> IPAGIIPTGNVLSTIEVCAHRCIFDFFKQIRSDDNSLYSAQFDILLGTYCNTLNFVRFLELGLSVACICTKFPELAYVRDGVIQFEVQQPMIARDGPHPVDQPVHNYMVKRIHKRSLSAAFAIASEALSLLSNTYVDGTEIDSSLRIRAIQQMARNLRTVSDSFERGTADQLLGVLLEKAPPLSLLSPINKFQPEGHLNRVARAALLSDLKRRVCADMFFMTRHAREPRLISAYLSDMVSCTQPSVMVSRITHTNTRGRQVDGVLVTTATLKRQLLQGILQIDDTAADVPVTYGEMVLQGTNLVTALVMGKAVRGMDDVARHLLDITDPNTLNIPSIPPQSNSDSTTAGLPVNARVPADLVIVGDKLVFLEALERRVYQATRVAYPLIGNIDITFIMPMGVFQANSMDRYTRHAGDFSTVSEQDPRQFPPQGIFFYNKDGILTQLTLRDAMGTICHSSLLDVEATLVALRQQHLDRQCYFGVYVAEGTEDTLDVQMGRFMETWADMMPHHPHWVNEHLTILQFIAPSNPRLRFELNPAFDFFVAPGDVDLPGPQRPPEAMPTVNATLRIINGNIPVPLCPISFRDCRGTQLGLGRHTMTPATIKAVKDTFEDRAYPTIFYMLEAVIHGNERNFCALLRLLTQCIRGYWEQSHRVAFVNNFHMLMYITTYLGNGELPEVCINIYRDLLQHVRALRQTITDFTIQGEGHNGETSEALNNILTDDTFIAPILWDCDALIYRDEAARDRLPAIRVSGRNGYQALHFVDMAGHNFQRRDNVLIHGRPVRGDTGQAIPITPHHDREWGILSKIYYYIVIPAFSRGSCCTMGVRYDRLYPALQAVIVPEIPADEEAPTTPEDPRHPLHAHQLVPNSLNVYFHNAHLTVDGDALLTLQELMGDMAERTTAILVSSAPDAGAATATTRNMRIYDGALYHGLIMMAYQAYDETIATGTFFYPVPVNPLFACPEHLASLRGMTNARRVLAKMVPPIPPFLGANHHATIRQPVAYHVTHSKSDFNTLTYSLLGGYFKFTPISLTHQLRTGFHPGIAFTVVRQDRFATEQLLYAERASESYFVGQIQVHHHDAIGGVNFTLTQPRAHVDLGVGYTAVCATAALRCPLTDMGNTAQNLFFSRGGVPMLHDNVTESLRRITASGGRLNPTEPLPIFGGLRPATSAGIARGQASVCEFVAMPVSTDLQYFRTACNPRGRASGMLYMGDRDADIEAIMFDHTQSDVAYTDRATLNPWASQKHSYGDRLYNGTYNLTGASPIYSPCFKFFTPAEVNTNCNTLDRLLMEAKAVASQSSTDTEYQFKRPPGSTEMTQDPCGLFQEAYPPLCSSDAAMLRTAHAGETGADEV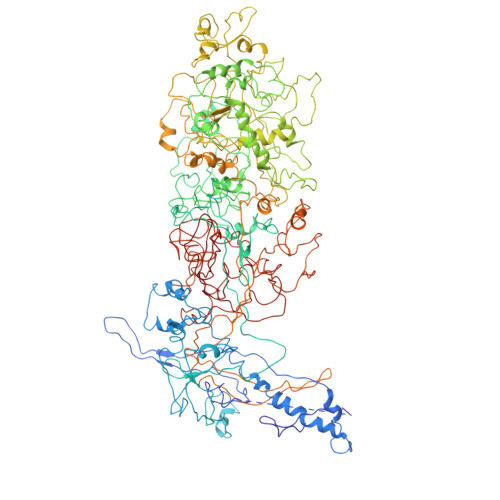HLAQYLIRDASPLRGCLPL> GMQAKGEAAMRDLIAELHAMQSPYTVQRFISSGSYGAVCAGVDSEGIPVAIKRVFNTVSDGRTVNILSDSFLCKRVLREIRLLNHFHHPNILGLRDIFVHFEEPAMHKLYLVTELMRTDLAQVIHDQRIVISPQHIQYFMYHILLGLHVLHEAGVVHRDLHPGNILLADNNDITICDFNLAREDTADANKTHYVTHRWYRAPELVMQFKGFTKLVDMWSAGCVMAEMFNRKALFRGSTFYNQLNKIVEVVGTPKIEDVVMFSSPSARDYLRNSL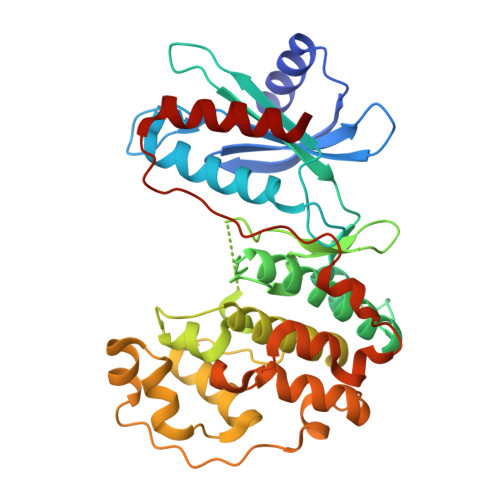SNVPARAWTAVVPTADPVALDLIAKMLEFNPQRRISTEQALRHPYFESLFDPLDLTEGLSERFHFDESVTDVYDMHKIFTAEVERFND>[2x]MRPYYIAIVGSGPSAFFAAASLLKAADTTEDLDMAVDMLEMLPTPWGLVRSGVAPDHPKIKSISKQFEKTAEDPRFRFFGNVVVGEHVQPGELSERYDAVIYAVGAQSDRMLN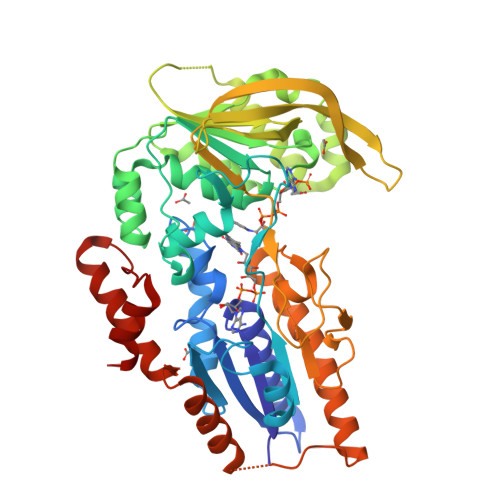IPGEDLPGSIAAVDFVGWYNAHPHFEQVSPDLSGARAVVIGNGNVALDVARILLTDPDVLARTDIADHALESLRPRGIQEVVIVGRRGPLQAAFTTLELRELADLDGVDVVIDPAELDGITDEDAAAVGKVCKQNIKVLRGYADREPRPGHRRMVFRFLTSPIEIKGKRKVERIVLGRNELVSDGSGRVAAKDTGEREELPAQLVVRSVGYRGVPTPGLPFDDQSGTIPNVGGRINGSPNEYVVGWIKRGPTGVIGTNKKDAQDTVDTLIKNLGNAKEGAECKSFPEDHADQVADWLAARQPKLVTSAHWQVIDAFERAAGEPHGRPRVKLASLAELLRIGLG> SAHNAYNAGIMQKTGKAFADEFFAEENQVVHESNAVVLVLMKSDEIDAIIEDIVLKGGKAKNPSIVVEDKAGFWWIKADGAIEIDAAEAGELLGKPFSVYDLLIGVSATVGRAYTLGTKFTITSELMGLDRA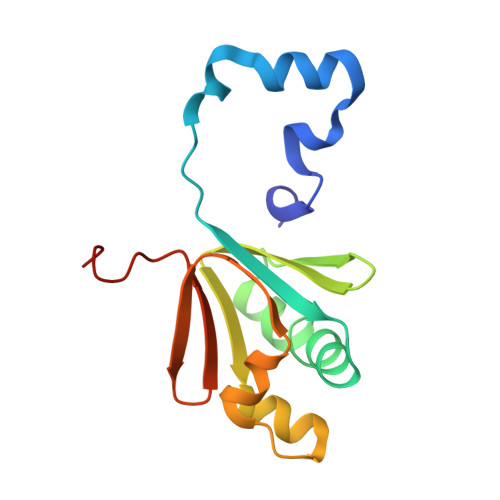LTDI> MLKRIKIVTSLLLVLAVFGLLQLTSGGLFFNALKNDKENFTVLQTIRQQQS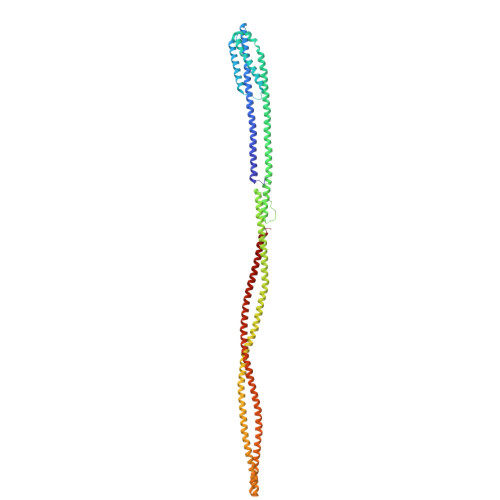TLNGSWVALLQTRNTLNRAGIRYMMDQNNIGSGSTVAELMESASISLKQAEKNWADYEALPRDPRQSTAAAAEIKRNYDIYHNALAELIQLLGAGKINEFFDQPTQGYQDGFEKQYVAYMEQNDRLHDIAVSDNNASYSQAMWILVGVMIVVLAVIFAVWFGIKASLVAPMNRLIDSIRHIAGGDLVKPIEVDGSNEMGQLAESLRHMQGELMRTVGDVRNGANAIYSGASEIATGNNDLSSRTEQQAASLEETAASMEQLTATVKQNAENARQASHLALSASETAQRGGKVVDNVVQTMRDISTSSQKIADIISVIDGIAFQTNILALNAAVEAARAGEQGRGFAVVAGEVRNLAQRSAQAAREIKSLIEDSVGKVDVGSTLVESAGETMAEIVSAVTRVTDIMGEIASASDEQSRGIDQVGLAVAEMDRVTQQNAALVEESAAAAAALEEQASRLTEAVAVFR[(2~{S})-3-(1~{H}-imidazol-4-yl)-2-[[2-methyl-3-oxidanyl-5-(phosphonooxymethyl)pyridin-4-yl]methylamino]propyl] dihydrogen phosphate | C14 H22 N4 O9 P2 | 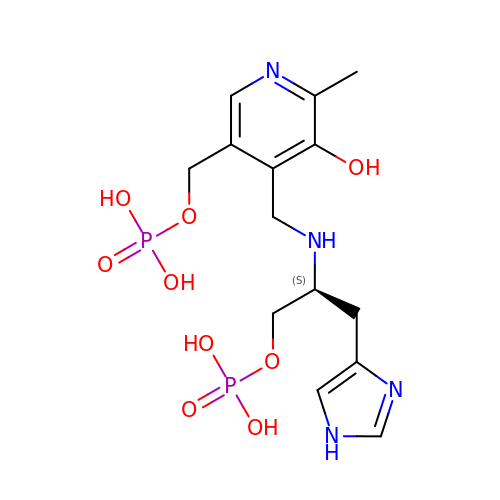WJUXYPJSYWWQCX-LBPRGKRZSA-N A common step during their assembly is polyketide trimming, which Afyg1p, Wdyg1p, and PlAntI catalyze. In summary, the N‐ and C‐domains in all three enzymes are oriented in a back‐to‐back fashion forming an interface that encloses the intramolecular binding cavity next to the active site. The catalytic triad is formed exclusively by the α/β‐hydrolase domain with the nucleophilic serine located in the consensus GXSXG esterase motif. The resulting Ser‐His‐Asp network is perfectly aligned with distances in the range of 2.5–2.8 Å between the active‐site residues.

For example, in Aspergillus fumigatus (Af), the type I PKS AfPksP produces the naphthopyrone heptaketide YWA1, whose acetoacetyl side chain is removed by the serine hydrolase Afyg1p. Single‐wavelength anomalous diffraction (SAD) was performed to obtain experimental phases for Afyg1p, which was used as a model for Patterson search calculations of the Wdyg1p structure. Both enzymes consist of an N‐domain and a C‐domain connected with a short linker. The N‐domains exhibit an α‐helix bundle, whereas the C‐domains adopt a classical α/β‐hydrolase topology. The amino acid sequences of Afyg1p and Wdyg1p have 40% sequence identity, which explains the similarity in their overall folds and active‐site residues (rmsd = 1.1 Å over 382 Cα‐atoms, Figure 3b). Although both enzymes differ significantly from PlAntI in terms of catalysis and primary sequence, their superposition shows a perfect match of secondary structure elements (rmsd = 1.6 Å over 244 Cα‐atoms for Afyg1p and rmsd = 1.8 Å over 247 Cα‐atoms for Wdyg1p). Consistent with the more extended polar substrate, the acetoacetyl binding site in Afyg1p is less hydrophobic, and the chamber formed by Ala258, Tyr287, Ile305, Trp309, and Val355 is increased in size (800 Å3). Thereby, Trp309 is located adjacent to the oxyanion hole and coordinates a well‐defined water molecule that is also present in Afyg1papo, Afyg1pPMSF, and Afyg1p:1,3‐DHN, as well as in Afyg1p:THN. Thus, the indole group of Trp309 likely stabilizes the distal carbonyl oxygen atom in the acetoacetyl sidechain. Taken together, the specificity pocket of Afyg1p is entirely occupied by the product, whereas in Afyg1papo, each position matching the hydroxyl groups 1─OH, 6─OH, and 8─OH of THN and 1─OH of 1,3‐DHN (analogous to 3─OH in THN) is filled by a water molecule.

>MRGSHHHHHHENLYFQGSPRWILGDKFDTVFPHKGSLKVLWESRWKFACSKSVYPFHDGSIEDFEPIFNHLISKNINDAASDEYTQAFLPTASALEEKAAQALQAGKHEEASNLLCRAAVVYRISRFPYVDITKPNSIKRVAFERQKQAYLKATSLWTQPIREVTVPHTYRTGNDGAHIPIYIRTPAGADQSNPVPIVLIMTGLDGYRPDNSQRTHEILARGWAAVVAEIPGTADCPADPADPASPDRLWDSVLSYLDQRPELNTAKMVVWGLSAGGYYAIRAAHTHRDRLLGAIAHGPGCHYYLDPEWLAKVNDHEYPFEITAAWATKHGYKTVEEFVAGAQKKFSLVETGIVDQPSCRLLLLNGVDDGVVPIEDCLVLFEHGSPKEGRFYKGLPHMGYPNSLPVSYEWLEQVLASPSKTKN[4x]The attachment of the ubiquitin-like protein ISG15 to substrates by specific E1-E2-E3 enzymes is a well-established signalling mechanism of the innate immune response. The enzymes responsible for ISG15 conjugation were first described over 15 years ago and include: the E1 activating enzyme UBE1L/UBA7, the E2 conjugating enzyme UBE2L6/UbcH8, and the HECT E3 ligase HERC5. In a multi-step process, ISG15 is first activated or adenylated by UBE1L, then sequentially transferred to the catalytic cysteines of the E1-E2-E3 enzymes, and targeted to substrate lysine residues. Reminiscent of linear diubiquitin, ISG15 is composed of two ubiquitin-like domains fused together through a short linker sequence.

Using cryo-EM, we obtained a 3.45 Å structure of the UBE1L-UBE2L6-ISG15 complex. Using a chemical biology approach which allows the capture of these transient reaction intermediates, we cross-link the active sites of UBE1L and UBE2L6 to form a multiprotein complex assembly. To prevent non-specific crosslinking, the non-catalytic UBE2L6 cysteine residues were mutated to serine (UBE2L6C86only), which was also utilized for UBE2L6 in a recent publication by Olsen and colleagues. Similar to other E1 enzymes, and as seen in a related study published while our paper was in revision, the UBE1L structure consists of four distinct domains: the adenylation domain (AD; which contains both the inactive adenylation domain & active adenylation domain), first catalytic cysteine half domain (FCCH), second catalytic cysteine half domain (SCCH) and ubiquitin-fold domain (UFD). The adenylation domain, which activates ISG15 via ATP-dependent adenylation of the C-terminal glycine, forms the largest contact surface with ISG15. Interestingly, we observed density extending from ISG15’s C-terminus into the adenylation active site, indicating the ISG15 C-terminal glycine is adenylated in our structure. ISG15 is located at the center of the complex, with multiple UBE1L domains cradling the C-terminal ubiquitin-like fold (C-lobe). Interestingly, the N-terminal ubiquitin-like fold (N-lobe) is not visible in the cryo-EM density, presumably due to its flexibility during the adenylation reaction. As anticipated, the active site cysteines of the SCCH domain and UBE2L6 were located within proximity for disulfide bond formation. The last domain, the UFD, adopts a well-characterized binding mode for E1-mediated E2 recruitment, where the UFD engages the N-terminal helix of UBE2L6.

> GSMDALDASKLLDEELYSRQLYVLGSPAMQRIQGARVLVSGLQGLGAEVAKNLVLMGVGSLTLHDPHPTCWSDLAAQFLLSEQDLERSRAEASQELLAQLNRAVQVVVHTGDITEDLLLDFQVVVLTAAKLEEQLKVGTLCHKHGVCFLAADTRGLVGQLFCDFGEDFTVQDPTEAEPLTAAIQHISQGSPGILTLRKGANTHYFRDGDLVTFSGIEGMVELNDCDPRSIHVREDGSLEIGDTTTFSRYLRGGAITEVKRPKTVRHKSLDTALLQPHVVAQSSQEVHHAHCLHQAFCALHKFQHLHGRPPQPWDPVDAETVVGLARDLEPLKRTEEEPLEEPLDEALVRTVALSSAGVLSPMVAMLGAVAAQEVLKAISRKFMPLDQWLYFDALDCLPEDGELLPSPEDCALRGSRYDGQIAVFGAGFQEKLRRQHYLLVGAGAIGCELLKVFALVGLGAGNSGGLTVVDMDHIERSNLSRQFLFRSQDVGRPKAEVAAAAARGLNPDLQVIPLTYPLDPTTEHIYGDNFFSRVDGVAAALDSFQARRYVAARCTHYLKPLLEAGTSGTWGSATVFMPHVTEAYRAPASAAASEDAPYPVCTVRYFPSTAEHTLQWARHEFEELFRLSAETINHHQQAHTSLADMDEPQTLTLLKPVLGVLRVRPQNWQDCVAWALGHWKLCFHYGIKQLLRHFPPNKVLEDGTPFWSGPKQCPQPLEFDTNQDTHLLYVLAAANLYAQMHGLPGSQDWTALRELLKLLPQPDPQQMAPIFASNLELASASAEFGPEQQKELNKALEVWSVGPPLKPLMFEKDDDSNFHVDFVVAAASLRCQNYGIPPVNRAQSKRIVGQIIPAIATTTAAVAGLLGLELYKVVSGPRPRSAFRHSYLHLAENYLIRYMPFAPAIQTFHHLKWTSWDRLKVPAGQPERTLESLLAHLQEQHGLRVRILLHGSALLYAAGWSPEKQAQHLPLRVTELVQQLTGQAPAPGQRVLVLELSCEGDDEDTAFPPLHYEL;> MGWDLTVKMLAGNEFQVSLSSSMSVSELKAQITQKIGVHAFQQRLAVHPSGVALQDRVPLASQGLGPGSTVLLVVDKSDEPLSILVRNNKGRSSTYEVRLTQTVAHLKQQVSGLEGVQDDLFWLTFEGKPLEDQLPLGEYGLKPLSTVFMNLRLRGG;> GPMMASMRVVKELEDLQKKPPPYLRNLSSDDANVLVWHALLLPDQPPYHLKAFNLRISFPPEYPFKPPMIKFTTKIYHPNVDENGQICLPIISSENWKPSTKTSQVLEALNVLVNRPNIREPLRMDLADLLTQNPELFRKNAEEFTLRFGVDRPS>MKKSLIALTTALSFGLAAAQTAAPVSAPQVPALTDVPAGHWAKDAIDRLVSRGVILGYPDGTFRGTQNLTRYEAAIIIARLLDQMRDGETPAGMTAEDMTALQNAIQELAADLAALGVRVSDLEANAVSKDDFARLEARIEEVAAAGGEQGATEALQGQIDDLTARVDEYDALRADVDDNASSIAALNDLTVLLNQDILDLQDRVSAVEAAQADFVQRSDFDALGGRVTTVETRVETVNNSLTGRIAALERNAFSVKPSLTIGYSVSRTSRNFDVDRLFPLNADGTVANNAFTSGGIDTDTGAQRRDFGDFGNASDPVVAGAAGLYGFADGVSYTVYFTDGSTATFDGLNPADYKVPTGKVIDTTKGRNGFGFNNLARYKEGSTDIGISLGFDTSGQFSQVTSGTGGSLFSTAGRLQVNQIDLNFGLVTGLPSDAYVDTNGNGKKDDGEATGRGTYLGSGGTAAILRDPAGNVYRPVFFRFKNATTQFSVGNNPVIVTLGQQQKFYFSDYVFDNNYDGRGDGFTVTVDGSNVPVIGAWKPQIKGVYGSRSGLDGTAEAGYGVYYRGVRAQITPVGTLTAGIHYAQEGRDMFGAAQNTTSTPSDVTTYGADLHGKAFGVELHSEYATSRVRPNTANAAVQTSNAFYARVATRKDNLAFDLNTPAAKFGNDTFGVSLYDLNYRKIDAGYNNVAGISEYGYGSYSRTSAQNIAYNPDTGVTAPFANLDRQAYTDANNDGTSDRNADGTVVATNTKIGQMGFGVKAAANLGPVAIGGYYDTSTGANGDNANRMTEAGGSAKVAYSIFSLRGTYNTLDSNRPQIYRDAAGTQIIGDAKVRRYAVQADVTPGLGLFVGAYYRDVNVNGVRSTTDRGLLGRGYLASSFEPGVGNNAYRTGLRCADNNFGTGTRDIDGVGGVLNPAVNLDQSRTATCFTSYGVEAGHAGDNANALVKDLFFRVGYSRVYVPTTATATTGDFSGSVTYGDARYDRKVGVANVRLAGSFSTTNTQLDSRPAGTRGAVGLIVRTDPLENVPFRPQFNGQVGYYTADNRVAAGNYNANATKYGAGVVLNDFLLPQTKIGVRYDGYMAQNRQYTPFDGDGTQGYFSDANNNRRTNLNGVYVEGAYQDLIFSYGTYTLSQKDLNGVEYGSGINNGQPARGQTFKISYKVNF[3x]

We have solved the atomic structure of a highly abundant protein, SlpA, and discovered that it forms extended structures that link the outer membrane (OM) to the peptidoglycan (PG). Our structure shows that SlpA exhibits a tripartite organization, with its C-terminal part forming a homotrimeric 30-stranded OM β-barrel (OMBB), its central part forming a trimeric coiled coil that can traverse the large periplasmic space, and the extreme N-terminal part forming an SLH domain trimer that can interact with the PG layer. Our results indicate that SlpA cannot fully tile the OM and that it is not a fundamental component of the S-layer, but that it connects the OM to the PG layer by forming extended homotrimers. Deletion of slpA leads to substantial disruption of the D. radiodurans cell envelope, suggesting its important role in the maintenance of cell envelope integrity.

We performed single-particle analysis on this cryo-EM data to solve a global 3.3-Å resolution structure of SlpA, with the best resolution in the β-barrel of 2.9 Å at the core. The structure showed that SlpA forms a homotrimer of 30-antiparallel–stranded β-barrels (30 β-strands per SlpA monomer). The SlpA β-barrel is the first structurally characterized 30-stranded barrel and one of the largest single-chain β-barrels observed. The C-terminal OMBB of the D. radiodurans SlpA is preceded by a long, homotrimeric coiled-coil segment, which, in our cryo-EM map, is well resolved from residue 215 onwards. When compared to its homologs, the OMBB of D. radiodurans SlpA (residues 254 to 1167) contains several insertions positioned within the pore. Residues 272 to 377 form the most extensive, ordered insertion that lines the cavity of the pore. This insertion appears to be stabilized by a canonical bacterial SLP metal ion–binding site coordinated by residues D274, D276, and D310. Although density for metal ions is resolved in our cryo-EM map, the identity of the metal is unknown. The protein:protein interface of the SlpA β-barrel consists mainly of stacked β-sheets from apposing barrels. These sheets contain a hydrophobic patch made up of residues L260, I262, Y264, I386, I388, L390, and F392 stacking onto V401, F479, F481, F488, and L499 from the next subunit. The coiled coil consists of a highly conserved, prominent salt bridge between E232 and R227.2-(2-HYDROXY-5-METHOXY-PHENYL)-1H-BENZOIMIDAZOLE-5-CARBOXAMIDINE 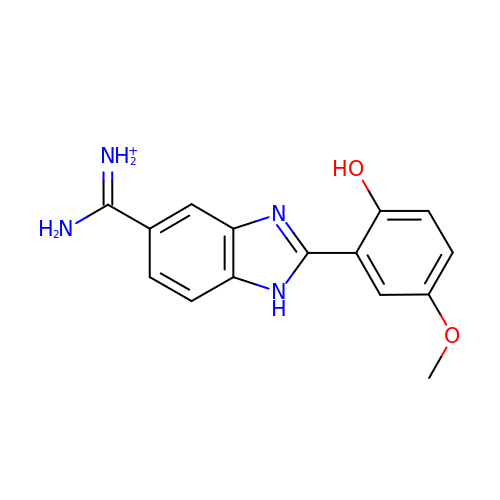| C15 H15 N4 O2 | ZFCKHJJALHETHG-UHFFFAOYSA-O>[2x]GSHMSDTTIVTVDHKDFDRTEKYLAEHFQLQNVDKADGHLMINAQKNYQVI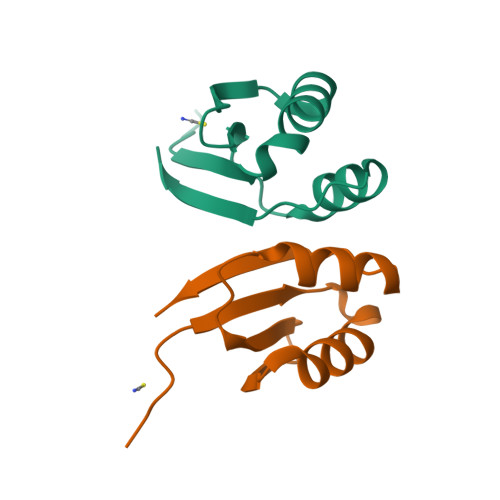LKALSELDIYPKYIETRKS>[5x]MFSGIKGPNPSDLKGPELRILIVHARWNLQAIEPLVKGAVETMIEKHDVKLENIDIESVPGSWELPQGIRASIARNTYDAVIGIGVLIKGSTMHFEYISEAVVHGLM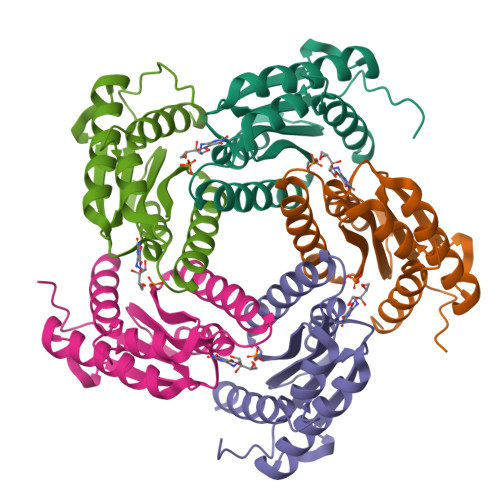RVGLDSGVPVILGLLTVLNEEQALYRAGLNGGHNHGNDWGSAAVEMGLKALY>[2x]MAAQKSPQDMDRFIDALMKKMTVEEKIGQLNLPVTGEIT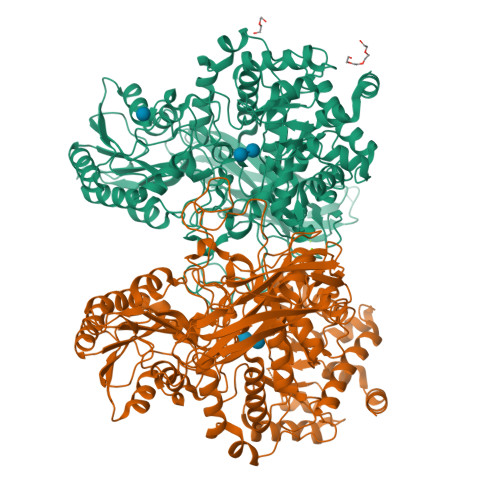TGQAKSSDIAAKIKRGEVGGLFNLKGVEKIRDVQKQAVEQSRLGIPLLFGMDVIHGYETMFPIPLGLSCTWDMTAIEESARIAAIEASADGISWTFSPMVDISRDPRWGRVSEGSGEDPFLGAMIAEAMVLGYQGKDMQRNDEIMACVKHFALYGAGEGGRDYNTVDMSRQRMFNEYMLPYEAAVEAGVGSVMASFNEVDGVPATANKWLMTDVLRGQWGFNGFVVTNYTGISEMIDHGIGDLQTVSARAINAGVDMDMVSEGFVSTLKKSIQEGKVSMETLNTACRRILEAKYKLGLFDNPYKYCDLKRPARDIFTKAHRDAARRIAAESFVLLKNDNVTLRPGTPAEPLLPFNPKGNIAVIGPLADSRTNMPGTWSVAAVLDRCPSLVEGLKEMTAGKANILYAKGSNLISDASYEERATMFGRSLNRDNRTDEQLLNEALTVANQSDIIIAALGESSEMSGESSSRTDLNIPDVQQNLLKELLKTGKPVVLVLFTGRPLTLTWEQEHVPAILNVWFGGSEAAYAIGDALFGYVNPGGKLTMSFPKNVGQIPLYYAHKNTGRPLAQGKWFEKFRSNYLDVDNEPLYPFGYGLSYTTFSYGDIDLSRSTIDMTGELTAAVMVTNTGTWPGSEVVQLYIRDLVGSTTRPVKELKGFQKIFLEPGQSEIVRFKIAPEMLRYYNYDLQLVAEPGEFEVMIGTNSRDVKSARFTLKLEHHHHHH>[8x]GPSGRNSSLSSVSGSTVAGDKIPIKTTHAALSWNSLKIGKSEIKEFTIRNTSNNKIKIQATISDSEKNFRFLRERETIGTTIVLALQGSESRTLSVVFSPHHIGAASGKIIFRHYQSKKEDSESLPSRQIFLYGYGGYSKVEISEVFKDTNGKMWLSFGMLNSENSLNAKIKLQNTGDLCSYVKIKLTPKAVYPTMISSWQVNPTELLLNPKEVQWVTLEFHPRKEDLALLQKSDVSHVGTLLITHGDEPTRLRIRRLYKKMKETGELNGNENETFRNIVHPICKVFSGEQLVSDVIPIRDSVQNFGDLCREIRQHEIMLTMEVCADETLTVLHDNPDESQ

Spd-2/CEP192 proteins, defined by a conserved “Spd-2 domain” (SP2D) comprising two closely spaced AspM-Spd-2-Hydin (ASH) domains, play a critical role in centrosome assembly. The conserved centriole/centrosome protein Spd-2/CEP192 (fly/human nomenclature) plays an important part in mitotic centrosome assembly in humans, flies, and worms and also in the diverged centrosomes of Dictyostelium, which lack canonical centrioles. In flies and worms, the phosphorylation of Spd-2/SPD-2 at centrioles recruits Polo/Polo-like kinase 1 (PLK1), which then phosphorylates the large coiled-coil protein Cnn/SPD-5 to stimulate the assembly of a Cnn scaffold, and the internal molecular interactions that allow Cnn and SPD-5 to assemble into scaffolds are beginning to be elucidated. ASH domains are present in several proteins associated with centrosomes, cilia, flagella, and the Golgi complex, but the functions of these domains remain largely unknown.

Despite extensive efforts, we were unable to crystallize DmSP2D, but we were able to crystallize the SP2D from the honeybee Apis dorsata and solved its structure to a resolution of 3.5 Å. Although side-chain visibility at this resolution is partly limited, the structure allowed its comparison to the human SP2D structure to reveal the underlying conserved interactions. Both structures adopt a very similar overall fold (252 Cα pairs with an RMSD of 2.27 Å). Thus, the extended cradle arrangement of the two ASH domains appears to be a conserved and defining feature of the SP2D. In both humans and honeybees, the extended cradle structure is assembled around a large insertion in the second ASH domain of the SP2D that loops out of the main β-sandwich to form a “bridge” that interacts with the first ASH domain and helps to hold the two ASH domains in their stereotypical conformation. This insertion consists of a short helix (α1) that emerges from β-f of the β-sandwich and extends as a less well-structured region that wraps around α1, enclosing a cluster of hydrophobic residues that form a stabilizing core (highlighted in red labels). In HsSP2D, Gln1995 in the α1 helix forms salt bridge interactions with Ser1876 via a nitrate ion trapped in a cavity, whereas in the AdSP2D, Arg1197 in the α1 helix forms salt bridge interactions with the side chain of Asp1244 and with the backbone-carbonyl oxygen of Trp976. Thus, although the stereospecific orientation of the two ASH domains in the SP2D is highly conserved, the internal molecular interactions that ensure their orientation appear to have partly diverged between humans and honeybees. Intriguingly, a similar crystal-packing interaction interface involving F1090 and W1098 was observed in the Apis Spd-2 SP2D crystal structure (cyan).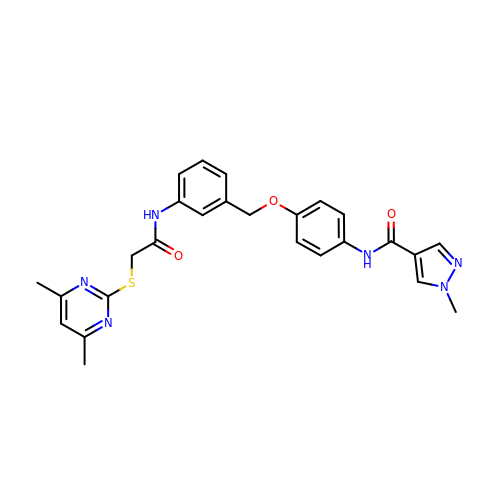N-[4-[[3-[2-(4,6-dimethylpyrimidin-2-yl)sulfanylethanoylamino]phenyl]methoxy]phenyl]-1-methyl-pyrazole-4-carboxamide | C26 H26 N6 O3 S | NPUWKDPBMLZNJM-UHFFFAOYSA-N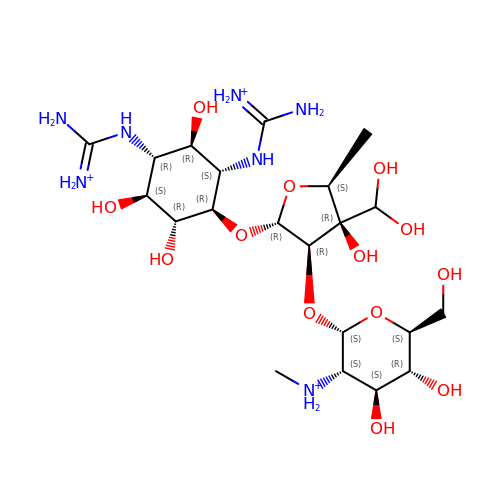[(2~{S},3~{S},4~{S},5~{R},6~{S})-2-[(2~{R},3~{R},4~{R},5~{S})-2-[(1~{R},2~{S},3~{R},4~{R},5~{S},6~{R})-2,4-bis[[azaniumylidene(azanyl)methyl]amino]-3,5,6-tris(oxidanyl)cyclohexyl]oxy-4-[bis(oxidanyl)methyl]-5-methyl-4-oxidanyl-oxolan-3-yl]oxy-6-(hydroxymethyl)-4,5-bis(oxidanyl)oxan-3-yl]-methyl-azanium | C21 H44 N7 O13 | ATLHDHNZEMANQF-UQHZJGBMSA-Q>[4x]SDKIIHLTDDSFDTDVLKADGAILVDFWAEWCA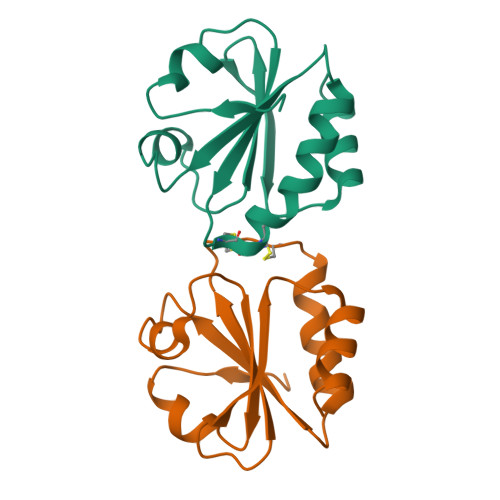CAKMIAPILDEIADEYQGKLTVAKLNIDQNPGTAPKYGIRGIPTLLLFKNGEVAATKVGALSKGQLKEFLDANLA>MRGSHHHHHHGSQKTSDLIVLGLPWKTTEQDLKEYFSTFGEVLMVQVKKDLKTGHSKGFGFVRFTEYETQVKVMSQRHMIDGRWCDCKLPNSKQSQDEPLRSR[2x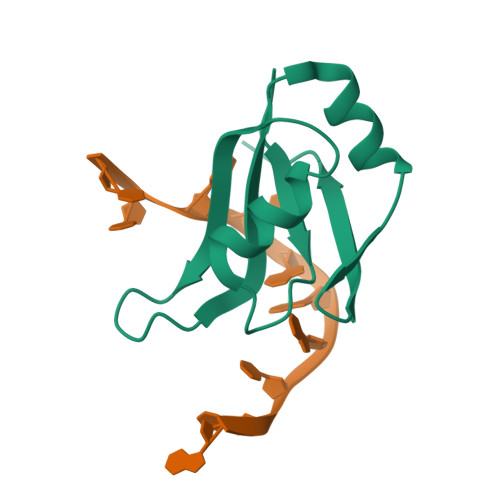]Transient receptor potential vanilloid (TRPV) channels are a group of six polymodal cation channels subdivided into two subgroups by their sequence identity and functional properties. TRPV1–TRPV4 comprise the first subgroup of non-selective Ca2+ channels, TRPV5 and TRPV6 constitute the second subgroup of Ca2+ selective channels. TRPV channels are blocked by ruthenium red (RR), a universal pore blocker for a wide array of cation channels. Here we use cryo-electron microscopy to reveal the molecular details of RR block in TRPV2 and TRPV5, members of the two TRPV subfamilies.

Next, we prepared cryo-EM grids of wild-type rabbit TRPV5 reconstituted into nanodiscs treated first with 400 μM PI(4,5)P2 for 5–10 min and then 1 mM RR for 45 min before preparing grids. This dataset yielded a single stable state: TRPV5PIP2+RR with C4 symmetry at 2.65 Å resolution. TRPV5PIP2+RR contained strong extra density at the TRPV5 SF consistent with the size and shape of RR, but did not show the expected density for PI(4,5)P2. The RR molecule in TRPV5PIP2+RR remains coordinated at Site 2, with the Thr539 backbone carbonyl and sidechain hydroxyl forming hydrogen bonds (3.1–3.2 Å) with ammonia groups of the top ruthenium atom. The bottom of the RR molecule now occupies Site 3, which allows for the formation of hydrogen bonds with Asn572 (2.9 Å). TRPV5PIP2+RR also has density coordinated at Asp542 which is significantly separated from the RR density and is likely caused by the coordination of an ion at this position. Conversely, the addition of RR to PI(4,5)P2-activated TRPV5 caused the channel to close and take on a conformation identical to TRPV5Apo. No density in the TRPV5PIP2+RR map was observed for the PI(4,5)P2 molecule, likely because the channel is closed. Based on our data, we propose that RR interaction with Asn572 at Site 3 may pull the S6 helix towards the central axis of the pore and closes the lower gate at Ile575. This closure would draw the key Arg584 residue away from the PI(4,5)P2 binding site, leading to the observed loss of PI(4,5)P2 binding.

>[4x]MGACPPKAKGPWAQLQKLLISWPVGEQDWEQYRDRVNMLQQERIRDSPLLQAAKENDLRLLKILLLNQSCDFQQRGAVGETALHVAALYDNLEAATLLMEAAPELAKEPALCEPFVGQTALHIAVMNQNLNLVRALLARGASVSARATGAAFRRSPHNLIYYGEHPLSFAACVGSEEIVRLLIEHGADIRAQDSLGNTVLHILILQPNKTFACQMYNLLLSYDEHSDHLQSLELVPNHQGLTPFKLAGVEGNTVMFQHLMQKRKHVQWTCGPLTSTLYDLTEIDSWGEELSFLELVVSSKKREARQILEQTPVKELVSFKWKKYGRPYFCVLASLYILYMICFTTCCIYRPLKLRDDNRTDPRDITILQQKLLQEAYVTHQDNIRLVGELVTVTGAVIILLLEIPDIFRVGASRYFGQTILGGPFHVIIITYASLVLLTMVMRLTNMNGEVVPLSFALVLGWCSVMYFARGFQMLGPFTIMIQKMIFGDLMRFCWLMAVVILGFASAFHITFQTEDPNNLGEFSDYPTALFSTFELFLTIIDGPANYSVDLPFMYCITYAAFAIIATLLMLNLFIAMMGDTHWRVAQERDELWRAQVVATTVMLERKMPRFLWPRSGICGYEYGLGDRWFLRVENHHDQNPLRVLRYVEAFKCSDKEDGQEQLSEKRPSTVESGMLSRASVAFQTPSLSRTTSQSSNSHRGWEILRRNTLGHLNLGLDLGEGDGEEVYHFTETSQVAPA>[3x]MENSKTEQVTGATGITQSTVTAPLPEAVSSLSLAPTVNALDPWVYLNQTEVPGGTFTVSSATQPGSVLLELEISPELNLYTSHLFRMYAGWSGGFSLKLLVAGNAFSAGKLIAAIIPPNIEVPNSAYLLTGFPHEILDFRTADSMEIIAPDIKNIDYHFRGDKLGKLVVMVYSPLRSTSADFEIEIKLTSAPLPDFKFTMLVPPIQNNALPIWSIPQAPPYSMVNPRSPLTPVVELYINSSYATCNHQLGRYTIYQGAIGNSTFNPSGAWTATCTAEAGSVTGNPNWRYALLDLPDNPTFDPTLPPVPRGFCDWGSGVKSGNKQHLVCFTGKKFAGGFQDVDAHMWDYGDNETVGLDNTYQRTIYISDPSLEKDAQYLVIPMGVSGAANDDTVQVAPNCYGSWDYAPTVAPPLGEQFVWFRSQLPASKTTTTSGVNSVPVNVNALMSPDLIRSAYASGFPLGKVALLDYVLFGGSVVRQFKLY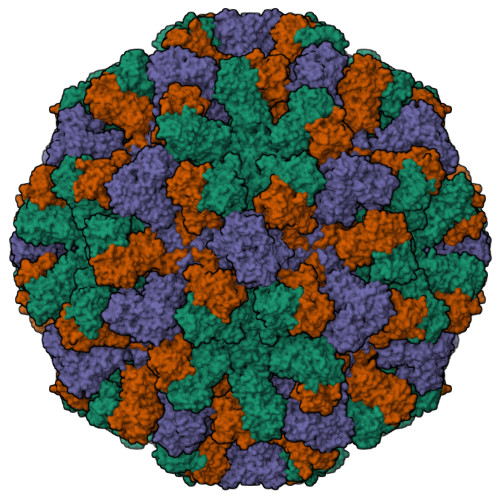PEGYMTANTTGSNTGFIIPADGYFRFNSWVSPSFMISSVVDLNLQTAVVFR2-{4-[(4'-METHOXYBIPHENYL-3-YL)SULFONYL]PIPERAZIN-1-YL}-3-(4-METHOXYPHENYL)PYRAZINE 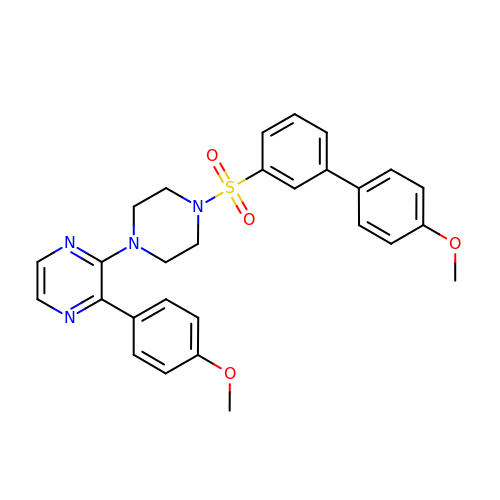| C28 H28 N4 O4 S | IQVDMFYVPSHFEP-UHFFFAOYSA-N>[8x]MAGKLMHALQYNSYGGGAAGLEHVQVPVPTPKSNEVCLKLEATSLNPVDWKIQKGMIRPFLPRKFPCIPATDVAGEVVEVGSGV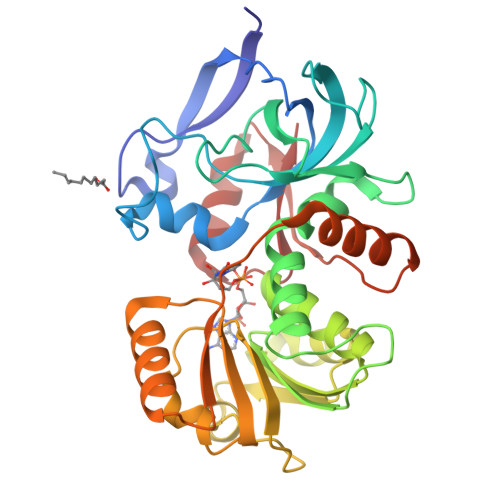KNFKAGDKVVAVLSHLGGGGLAEFAVATEKLTVKRPQEVGAAEAAALPVAGLTALQALTNPAGLKLDGTGKKANILVTAASGGVGHYAVQLAKLANAHVTATCGARNIEFVKSLGADEVLDYKTPEGAALKSPSGKKYDAVVHCANGIPFSVFEPNLSENGKVIDITPGPNAMWTYAVKKITMSKKQLVPLLLIPKAENLEFMVNLVKEGKVKTVIDSKHPLSKAEDAWAKSIDGHATGKIIVEP1-HYDROXY-3,7,11-TRIMETHYLDODECA-2,6,10-TRIENE PHOSPHONIC ACID | C15 H27 O4 P | 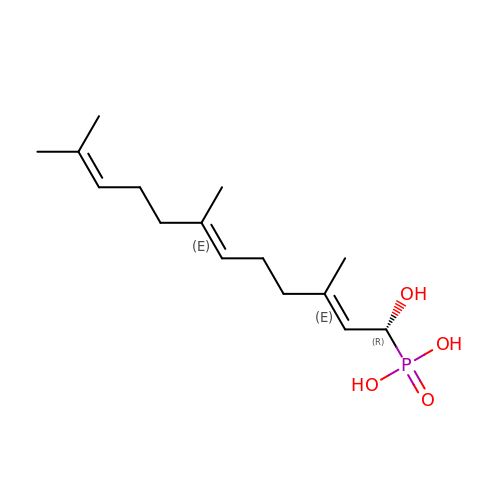MONZTFSZTWQCKH-UBHHKXJDSA-N>[2x]MPSYKLTYFFFRGLGEPIRLLFHLAGVQFEEVRMNPDQTWLDIKDSTPMKQLPVLNIDGFELPQSGAILRYLARKFGFAGKTPEEEAWVDAVHDLFKDFLAEFKKFAAERRSGKSAEEV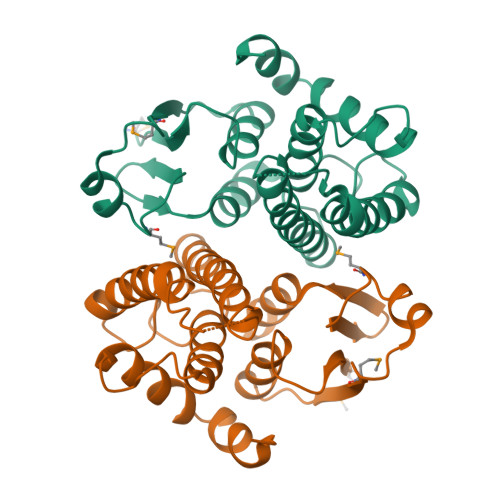EKFRSEFFLPARNTYFNILNGLLEKSNSGFLIGSDITFADLVVVDNLLTLKNYGLFDESEFTKLAALREKVNSYPGIKEYIAKRPVTEY> ATCDDGRTTANAACCILFPILDDIQENLFDGAQCGEEVHESLRLTFHDAIGFSPTLGGGGADGSIIAFDTIETNFPANAGIDEIVSAQKPFVAKHNISAGDFIQFAGAVGVSNCPGGVRIPFFLGRPDAVAASPDHLVPGPFDSVDSILARMGDAGFSPVEVVWLLASHSIAAADGVDPSIPGTPFDSTPEVFDSQFFIETQLKGRLFPGTADNKGEAQSPLQGEIRLQSDHLLARDPQTACEWQSMVNNQPKIQNRFAATMSKMALLGQDKTKLIDCSDVIPTPPALVGAAHLPA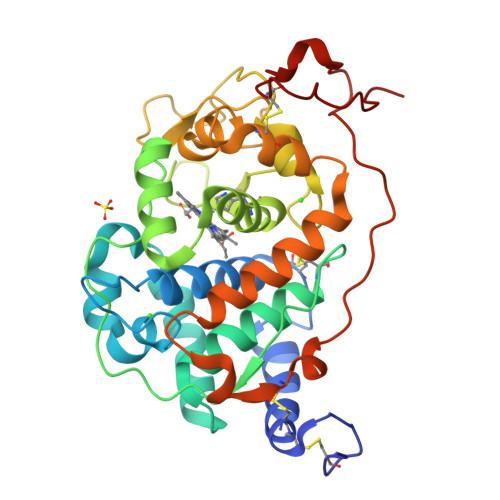GFSLSDVEQACAATPFPALTADP[2-AMINO-3-(4-HYDROXY-PHENYL)-PROPIONYLAMINO]- 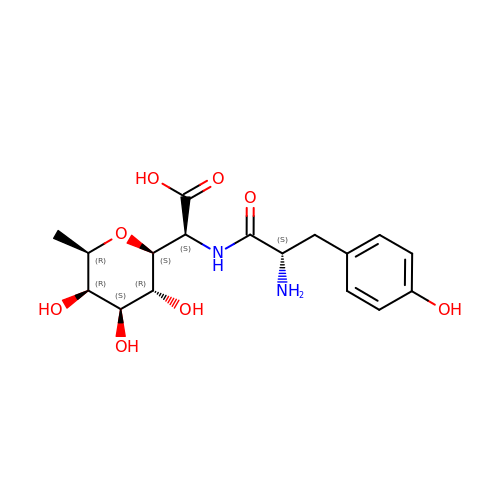(3,4,5-TRIHYDROXY-6-METHYL-TETRAHYDRO-PYRAN-2-YL)- ACETIC ACID | C17 H24 N2 O8 | KUCHJUZRDGYEDY-HRNUQJICSA-N(1R,2R,3S,4R,5R)-5-aminocyclopentane-1,2,3,4-tetrol | C5 H11 N O4 | 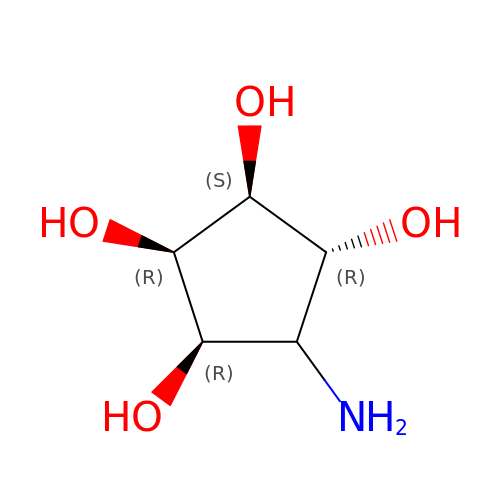LZCRRHQKPAEPKL-PTSYSAGVSA-N> GATAEKQKHDGRVKIGHYILGDTLGVGTFGKVKVGKHELTGHKVAVKILNRQKIRSLDVVGKIRREIQNLKLFRHPHIIKLYQVISTPSDIFMVMEYVSGGELFDYICKNGRLDEKESRRLFQQILSGVDYCHRHMVVHRDLKPENVLLDAHMNAKIADFGLSNMMSDGEFLRTSCGSPNYAAPEVISGRLYAGPEVDIWSSGVILYALLCGTLPFDDDHVPTLFKKICDGIFYTPQYLNPSVISLLKHMLQVDPMKRATIKDIREHEWFKQDLPKYLFPEDPSYSSTMIDDEALKEVCEKFECSEEEVLSCLYNRNHQDPLAVAYHLIIDNRRIMNEAKDFYLATSPPDSFLDDHHLTRPHPERVPFLVAETPRARHTLDELNPQKSKHQGVRKAKWHLGIRSQSRPNDIMAEVCRAIKQLDYEWKVVNPYYLRVRRKNPVTSTFSKMSLQLYQVDSRTYLLDFRSIDDEASGGPGGSAPRPGSHTIEFFEMCANLIKILAQ;> MEVNEKAPAQARPTVFRWTGGGKEVYLSGSFNNWSKLPLTRDQNNFVAILDLPEGEHQYKFFVD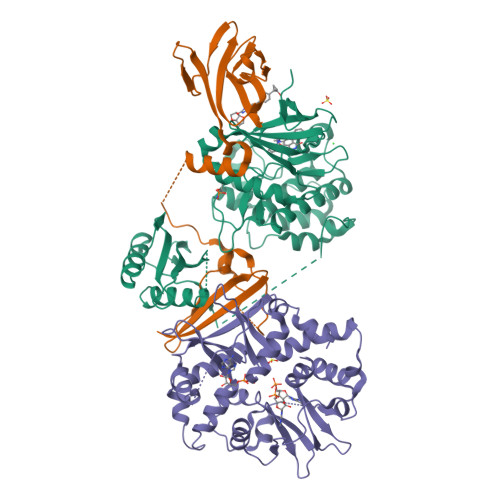GQWTHDPSEPIVTSQLGTVNNIIQVKKTDFEVFDALMVDSQKCSDVSELSSSPPGPYHQEPYISKPEERFKAPPILPPHLLQVILNKDTGISCDPALLPEPNHVMLNHLYALSIKDGVMVLSATHRYKKKYVTTLLYKPI;> MESVAAESAPAPENEHSQETPESNSSVYTTFMKSHRCYDLIPTSSKLVVFDTSLQVKKAFFALVTNGVRAAPLWDSKKQSFVGMLTITDFINILHRYYKSALVQIYELEEHKIETWREVYLQDSFKPLVCISPNASLFDAVSSLIRNKIHRLPVIDPESGNTLYILTHKRILKFLKLFITEFPKPEFMSKSLEELQIGTYANIAMVRTTTPVYVALGIFVQHRVSALPVVDEKGRVVDIYSKFDVINLAAEKTYNNLDVSVTKALQHRSHYFEGVLKCYLHETLEAIINRLVEAEVHRLVVVDEHDVVKGIVSLSDILQALVLTGGEKKP>[2x]QSASQFTDPTTGFQFTGITDPVHDVTYGFVFPPLATSGAQSTEFIGEVVAPIASKWIGIALGGAMNNDL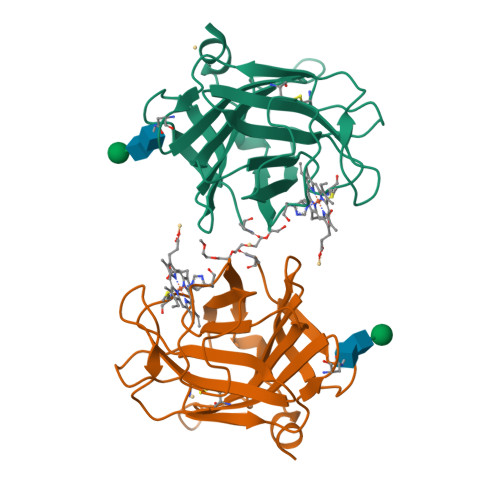LLVAWANGNQIVSSTRWATGYVQPTAYTGTATLTTLPETTINSTHWKWVFRCQGCTEWNNGGGIDVTSQGVLAWAFSNVAVDDPSDPQSTFSEHTDFGFFGIDYSTAHSANYQNYLN> GPHMSYQVLARKWRPQTFADVVGQEHVLTALANGLSLGRIHHAYLFSGTRGVGKTSIARLLAKGLNCETGITATPCGVCDNCREIEQGRFVDLIEIDAASRTKVEDTRDLLDNVQYAPARGRFKVYLIDEVHMLSRHSFNALLKTLEEPPEHVKFLLATTDPQKLPVTILSRCLQFHLKALDVEQIRHQLEHILNEEHIAHEPRALQLLARAAEGSLRDALSLTDQAIASGDGQVSTQAVSAMLGTLDDDQALSLVEAMVEANGERVMALINEAAARGIEWEALLVEMLGLLHRIAMVQLSPAALGNDMAAIE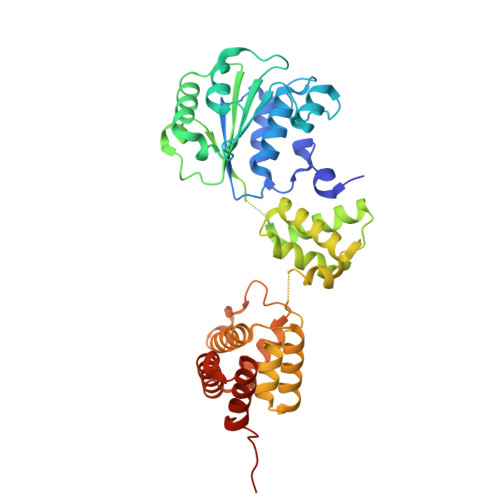LRMRELARTIPPTDIQLYYQTLLIGRKELPYAPDRRMGVEMTLLRALAFHPRMPLPEPEVPRQ>PENITLDTLNTQNDYEETHGESPEVPKASIAPAGRQNVPVLQQNQENKDNHALGGSEDAKDEREIRFSAIKTLYNYYSEGPSTPIMPHLVNRLRGLDALAKIDATLTKVDMNAAYIFALRPTFPYSYGYKQRFSNRRLTTSAVCYARTGLSSFLTVNKTYTSNSPLKGGSRGWPIFNVGVSPHVAEPHMRTLSPIGLEVFSQNLATFSKTLLTASSKVFTQSLYTADILSIFGEVFLPHVMQPVSNYTPILVRALLALIHILGPGSGNCSLSSSIFESSIPQFFTVSHSTNMSNRTRYCLHTWSAYKDMFRNGIPPQSTLPPTLAPEGSSARVLIPAALVTSPMFPWLLALVSSGPQFFLYSKDASINTVDIGSRGRITSPIPDVANLDLHRLWNLFRFDGHRYIDVVIVGVDRDYVWPYQNGVYVHGGKGPNGTDNYGNADVHDGIGTIFSSFNDNVNVQTSDLILGLLTLWNHITTTYATEEEVTMAIKIAAAFALVYPVQPIVYSGCPRAFQSHTSYYQPSSENCYTTDTAEVKSTWDTVELSVQVNNAMVLGMTLPFGQPTVSSAQWFNNIDKAEISMFKVGNLPLQNLDYLSLDMMEFYAPTTGQLYDIRSDNLILSAHRTVNLGIGYTALADFFAYLASVPAQSFYHDRMVTSPISKQTYSVYERFIERFVDDFVGWDRCDLFNLDTLLAAKRIAGVASSPIPWHCSLQRCPLPIIMHYTGLHFGQEHITVRDVAGVEGLQQIVMRNDQGKIVVDALGTAAPSRLAVKLDWSRLSAWYSDTTCAIPLSDRVMEIINYAAIWDPTQERRATGFVYTYFSPNFLSSFNASEPIFNTSINLTP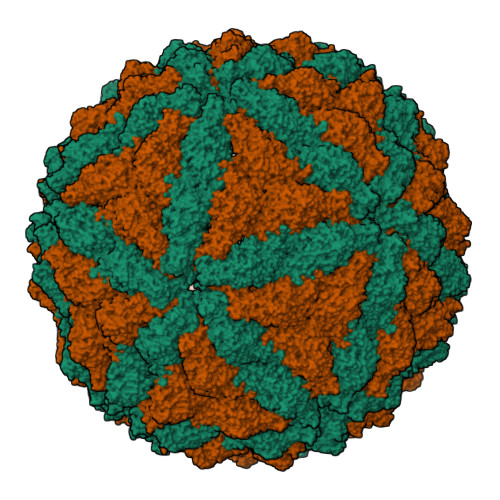PYDDTSHTVIQNLSMPQMLSFDPYYESTFYVVSADNEWIPTSGPAWKVPYLENVVKRSGRRLLAELRIASNNGSGDRTFLDDV[2x]>MAHNNENVSGISAYLLGLIIGDGGLYKLKYKGNRSEYRVVITQKSENLIKQHFAPLMQFLIDELNVKSKIQIVKGDTRYELRVSSKKLYYYFTNMLERIRLCNMREQIAFIKGLYVAEGDKTLKRLRIWNKNKALLEIVSRWLNNLGVRNTIHLDDHRHGVYVLNISL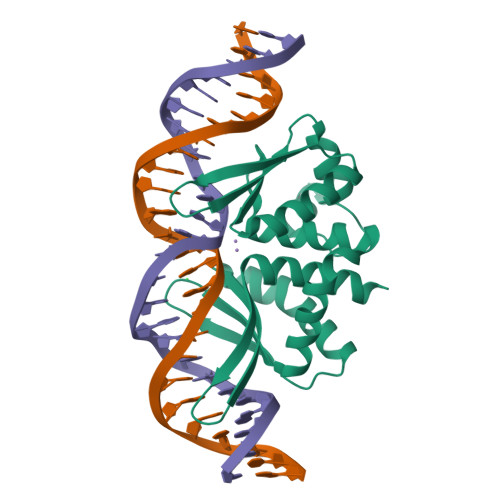RDRIKFVHTILSSHLNPLPPEAAALEHHHHHH[3x]>MARRLPKPTLQGRLEADFPDSPLLPKFQELNQNNLPNDVFREAQRSYLVFLTSQFCYEEYVQRTFGVPRRQRAIDKRQRASVAGAGAHAHLGGSSATPVQQAQAAASAGTGALASSAPSTAVAQSATPSVSSSISSLRAATSGATAAASAAAAVDTGSGGGGQPHDTAPRGARKKQ[5x];>MKVQGSVDRRRLQRRIAGLLPPPARRLNISRGSEFTRDVRGLVEEHAQASSLSAAAVWRAGLLAPGEVAVAGGGSGGGSFSWSGWRPPVFGDFLIHASSFNNAEATGTPLFQFKQSDPFSGVDAVFTPLSLFILMNHGRGVAARVEAGGGLTRMANLLYDSPATLADLVPDFGRLVADRRFHNFITPVGPLVENIKSTYLNKITTVVHGPVVSKAIPRSTVKVTVPQEAFVDLDAWLSGGAGGGGGVCFVGGLGLQPCPADARLYVALTYEEAGPRFTFFQSSRGHCQIMNILRIYYSPSIMHRYAVVQPLHIEELTFGAVACLGTFSATDGWRRSAFNYRGSSLPVVEIDSFYSNVSDWEVIL[2x];>[4x]MDLKVVVSLSSRLYTDEIAKMQQRIGCILPLASTHGTQNVQGLGLGQVYSLETVPDYVSMYNYLSDCTLAVLDEVSVDSLILTKIVPGQTYAIKNKYQPFFQWHGTGSLSVMPPVFGREHATVKLESNDVDIVFPMVLPTPIAEEVLQKILLFNVYSRVVMQAPGNADMLDVHMHLGSVSYLGHHYELALPEVPGPLGLALLDNLSLYFCIMVTLLPRASMRLVRGLIRHEHHDLLNLFQEMVPDEIARIDLDDLSVADDLSRMRVMMTYLQSLASLFNLGPRLATAAYSQETLTATCWLR;>[5x]MASNEGVENRPFPYLTVDADLLSNLRQSAAEGLFHSFDLLVGKDAREAGIKFEVLLGVYTNAIQYVRFLETALAVSCVNTEFKDLSRMTDGKIQFRISVPTIAHGDGRRPSKQRTFIVVKNCHKHHISTEMELSMLDLEILHSIPETPVEYAEYVGAVKTVASALQFGVDALERGLINTVLSVKLRHAPPMFILQTLADPTFTERGFSKTVKSDLIAMFKRHLLEHSFFLDRAENMGSGFSQYVRSRLSEMVAAVSGESVLKGVSTYTTAKGGEPVGGVFIVTDNVLRQLLTFLGEEADNQIMGPSSYASFVVRGENLVTAVSYGRVMRTFEHFMARIVDSPEKAGSTKSDLPAVAAGVEDQPRVPISAAVIKLGNHAVAVESLQKMYNDTQSPYPLNRRMQYSYYFPVGLFMPNPKYTTSAAIKMLDNPTQQLPVEAWIVNKNNLLLAFNLQNALKVLCHPRLHTPAHTLNSLNAAPAPRDRRETYSLQHRRPNHMNVLVIVDEFYDNKYAAPVTDIALKCGLPTEDFLHPSNYDLLRLELHPLYDIYIGRDAGERARHRAVHRLMVGNLPTPLAPAAFQEARGQQFETATSLAHVVDQAVIETVQDTAYDTAYPAFFYVVEAMIHGFEEKFVMNVPLVSLCINTYWERSGRLAFVNSFSMIKFICRHLGNNAISKEAYSMYRKIYGELIALEQALMRLAGSDVVGDESVGQYVCALLDPNLLPPVAYTDIFTHLLTVSDRAPQIIIGNEVYADTLAAPQFIERVGNMDEMAAQFVALYGYRVNGDHDHDFRLHLGPYVDEGHADVLEKIFYYVFLPTCTNAHMCGLGVDFQHVAQTLAYNGPAFSHHFTRDEDILDNLENGTLRDLLEISDLRPTVGMIRDLSASFMTCPTFTRAVRVSVDNDVTQQLAPNPADKRTEQTVLVNGLVAFAFSERTRAVTQCLFHAIPFHMFYGDPRVAATMHQDVATFVMRNPQQRAVEAFNRPEQLFAEYREWHRSPMGKYAAECLPSLVSISGMTAMHIKMSPMAYIAQAKLKIHPGVAMTVVRTDEILSENILFSSRASTSMFIGTPNVSRREARVDAVTFEVHHEMASIDTGLSYSSTMTPARVAAITTDMGIHTQDFFSVFPAEAFGNQQVNDYIKAKVGAQRNGTLLRDPRTYLAGMTNVNGAPGLCHGQQATCEIIVTPVTADVAYFQKSNSPRGRAACVVSCENYNQEVAEGLIYDHSRPDAAYEYRSTVNPWASQLGSLGDIMYNSSYRQTAVPGLYSPCRAFFNKEELLRNNRGLYNMVNEYSQRLGGHPATSNTEVQFVVIAGTDVFLEQPCSFLQEAFPALSASSRALIDEFMSVKQTHAPIHYGHYIIEEVAPVRRILKFGNKVVF

Epstein-Bar virus (EBV), a member of the subfamily gammaherpesviruses that also includes the Kaposi Sarcoma-associated herpesvirus (KSHV),2,3 is the first identified oncovirus. Similar to other members of the family herpesviridae, EBV has a characteristic three-layer configuration: the outer lipid bilayer envelope containing viral glycoproteins responsible for host recognizing and membrane fusion, the inner pseudo-icosahedral nucleocapsid enclosing a 172-kb double-strand DNA (dsDNA) genome and the middle pleomorphic tegument compartment fulfilled with 20–40 different viral proteins. All herpesvirus capsid shell consists of 4 abundant proteins: the major capsid proteins (MCP) constituting the basic capsid skeleton through forming 150 hexons and 11 pentons, the small capsid proteins (SCP) binding to the tops of hexon MCPs or both hexon and penton MCPs, and the Tri1 and Tri2 forming the heterotrimeric triplexes to plug the large holes on the capsid floor. Once the viral dsDNA genome enters the procapsid shell through the portal that is located at a unique 5-fold vertex of the icosahedral capsid, the viral nucleocapsid is joined by the capsid-associated tegument complexes (CATCs).

First, the dimerization domain of a penton MCP contains only a long helix and is unable to form type 2 interactions with the dimerization domain of a P1 MCP. Therefore, a penton MCP neither lashes a hexon MCP nor is lashed by a hexon MCP. Finally, the elbow-like helix-turn-helix structure in the buttress domain of a hexon MCP is instead a long straight helix in a penton MCP and directly contacts the MCP floor region to support the MCP tower. To analyze the CATC occupancy at the EBV penton vertices, we expanded the dataset of penton-vertex sub-particles with 5-fold symmetry and then performed focused 3D classification with a mask including only one CATC copy. We also identified 37.9% of the penton vertices in EBV are CATC-absent and obtained a reconstruction of the C5 CATC-absent penton vertex at 3.8 Å by 3D refinement. Intriguingly, compared to that of the CATC-binding triplex Ta, the main body of the CATC-absent triplex Ta is rotated ~120°, whereas their N-anchor regions essentially remain the same, which is also the case in KSHV. In contrast, the main bodies of both the CATC-absent and CATC-binding Ta in EBV exhibit ~120° rotations counterclockwise and clockwise, respectively. This finding indicates that the difference in conformation between the CATC-absent and CATC-binding Ta in EBV is not induced by CATC binding, but instead is predetermined, probably by the local curvature of the capsid floor as well as interactions with the surrounding MCPs. In addition, some of the penton vertices in both the KSHV (7.3%) and EBV (37.9%) mature nucleocapsids lack CATCs and thus remain vulnerable.>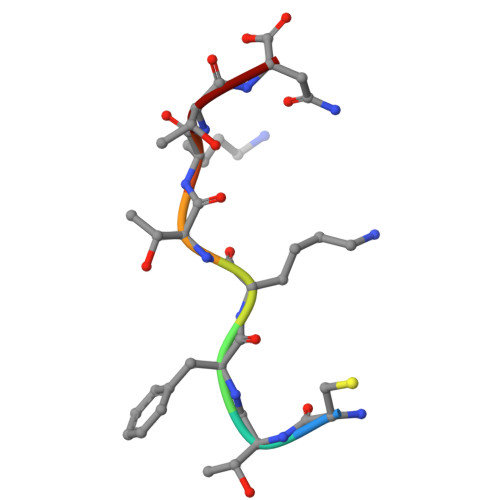 CTFKTKTN Clamp loaders are pentameric ATPases that place circular sliding clamps onto DNA, where they function in DNA replication and genome integrity. Because the sliding clamp is a closed ring in solution, it needs to be opened and placed onto DNA by a separate ATPase complex called the clamp loader. All clamp loaders are pentameric ATPases of the AAA + family (ATPases associated with various cellular activities). Here we describe a series of structures of the E. coli clamp loader in the process of placing the clamp onto a p/t-junction.

In micrographs of the sample containing ADP·BeFx, we observe two different conformations of the clamp loader/sliding clamp complex, both with the clamp open. However, the degree of opening is drastically different between these two states. In the first state, the clamp is barely opened and adopts a very tight spiral conformation (overall resolution = 3.9 Å). Therefore, we designate these two states as the Semi-Open and the Fully-Open states, respectively. Unlike the Initial-Binding complex, in the Semi-Open state, all five subunits of the clamp loader contact the sliding clamp. These additional contacts between the clamp loader and sliding clamp help stabilize the initial opening of the sliding clamp in a spiral conformation. Interface contacts between the A and B AAA+ modules and the C and D AAA+ modules are strong, while contacts between the B and C AAA+ modules remain minimal. In the Semi-Open state, there is a gap between the B and C subunits, which prevents the trans-acting arginine finger (Arg169 in γ, Arg158 in δ′) from interacting with ATP. The Semi-Open state, which was predicted by rapid kinetic studies, has all five AAA+ modules of the γ-complex gripping the ß-clamp. The AAA+ modules adopt a spiral matching the tight spiral of the clamp.

> MIRLYPEQLRAQLNEGLRAAYLLLGNDPLLLQESQDAVRQVAAAQGFEEHHTFSIDPNTDWNAIFSLCQAMSLFASRQTLLLLLPENGPNAAINEQLLTLTGLLHDDLLLIVRGNKLSKAQENAAWFTALANRSVQVTCQTPEQAQLPRWVAARAKQLNLELDDAANQVLCYCYEGNLLALAQALERLSLLWPDGKLTLPRVEQAVNDAAHFTPFHWVDALLMGKSKRALHILQQLRLEGSEPVILLRTLQRELLLLVNLKRQSAHTPLRALFDKHRVWQNRRGMMGEALNRLSQTQLRQAVQLLTRTELTLKQDYGQSVWAELEGLSLLLCH;>[3x]GPHMSYQVLARKWRPQTFADVVGQEHVLTALANGLSLGRIHHAYLFSGTRGVGKTSIARLLAKGLNCETGITATPCGVCDNCREIEQGRFVDLIEIDAASRTKVEDTRDLLDNVQYAPARGRFKVYLIDEVHMLSRHSFNALLKTLEEPPEHVKFLLATTDPQKLPVTILSRCLQFHLKALDVEQIRHQLEHILNEEHIAHEPRALQLLARAAEGSLRDALSLTDQAIASGDGQVSTQAVSAMLGTLDDDQALSLVEAMVEANGERVMALINEAAARGIEWEALLVEMLGLLHRIAMVQLSPAALGNDMAAIELRMRELARTIPPTDIQLYYQTLLIGRKELPYAPDRRMGVEMTLLRALAFHPRMPLPEPEVPRQ;> GPHMRWYPWLRPDFEKLVASYQAGRGHHALLIQALPGMGDDALIYALSRYLLCQQPQGHKSCGHCRGCQLMQAGTHPDYYTLAPEKGKNTLGVDAVREVTEKLNEHARLGGAKVVWVTDAALLTDAAANALLKTLEEPPAETWFFLATREPERLLATLRSRCRLHYLAPPPEQYAVTWLSREVTMSQDALLAALRLSAGSPGAALALFQGDNWQARETLCQALAYSVPSGDWYSLLAALNHEQAPARLHWLATLLMDALKRHHGAAQVTNVDVPGLVAELANHLSPSRLQAILGDVCHIREQLMSVTGINRELLITDLLLRIEHYLQPGVVLPVPHL;>[2x]GPHMKFTVEREHLLKPLQQVSGPLGGRPTLPILGNLLLQVADGTLSLTGTDLEMEMVARVALVQPHEPGATTVPARKFFDICRGLPEGAEIAVQLEGERMLVRSGRSRFSLSTLPAADFPNLDDWQSEVEFTLPQATMKRLIEATQFSMAHQDVRYYLNGMLFETEGEELRTVATDGHRLAVCSMPIGQSLPSHSVIVPRKGVIELMRMLDGGDNPLRVQIGSNNIRAHVGDFIFTSKLVDGRFPDYRRVLPKNPDKHLEAGCDLLKQAFARAAILSNEKFRGVRLYVSENQLKITANNPEQEEAEEILDVTYSGAEMEIGFNVSYVLDVLNALKCENVRMMLTDSVSSVQIEDAASQSAAYVVMPMRL V-ATPases function as proton pumps in acidic organelles and plasma membranes of eukaryotic cells. Furthermore, E. hirae V-ATPase physiologically functions as an ion pump, similar to eukaryotic V-ATPases34353637, and is composed of nine subunits with amino acid sequences that are homologous to those of the corresponding subunits of eukaryotic V-ATPases638. Thus, the V1 motor achieves its rotational dynamics via several conformational changes that are generated by the binding of ATP, release of Pi and ADP, and cooperative coupling among these conformational changes.

Next, we soaked the eV1 crystals in a high concentration (2 mM) of ADP to verify nucleotide binding to the third ‘bindable-like' form of 2ADPV1, and obtained the crystal structure (denoted 3ADPV1) at a resolution of 3.0 Å. Three ADP:Mg2+ molecules were bound at all three nucleotide-binding sites and induced conformational changes with the crystal packing rearrangements. We thus designated the unique half-closed AHCBO'' pair of 3ADPV1 as the ‘half-closed' form. A strong electron density peak for Pi or SO42− (a Pi analog) was observed at the nucleotide-binding site with ADP:Mg2+. In contrast, the DF axis and ‘ADP-bound' forms were slightly attracted to the AHC of the ‘half-closed' form. The shifted ‘ADP-bound' form was rather more similar to the observed ‘tight' conformation. We, therefore, designated this shifted ‘ADP-bound' form of 3ADPV1 as the ‘tight-like' form. The distances between the β-phosphate of ADP and the interacting residues in the ‘tight-like' form were slightly longer than those in the ‘ADP-bound' form, suggesting that the binding affinity for ADP of the ‘tight-like' form is lower than that of the ‘ADP-bound' form. Therefore, we inferred that the structure of 3ADPV1 corresponds to the state of waiting for ADP release (that is, ADP-release dwell) in the rotation. The DF axis of 3ADPV1 was slightly bent towards the ‘tight-like' form, but did not induce any rotational changes.

>GSSGSSGMQIGKIIKVSGPLVMAENMSEASIQDMCLVGDLGVIGEIIEMRQDVASIQVYEETSGIGPGEPVRSTGEALSVELGPGIISQMFDGIQRPLDTFMEVTQSNFLGRGVQLPALDHEKQWWFEATIEEGTEVSAGDIIGYVDETKIIQHKIMVPNGIKGTVQKIESGSFTIDDPICVIETEQGLKELTMMQKWPVRRGRPIKQKLNPDVPMITGQRVIDTFFPVTKGGAAAVPGPFGAGKTVVQHQIAKWSDVDLVVYVGCGERGNEMTDVVNEFPELIDPNTGESLMERTVLIANTSNMPVAAREASIYTGITIAEYFRDMGYDVAIMADSTSRWAEALREMSGRLEEMPGDEGYPAYLGSRLAEYYERSGRVIALGSDQREGSITAISAVSPSGGDISEPVTQNTLRVVKVFWGLDSSLAQKRHFPSINWIQSYSLYSTEVGRYMDQILQQDWSDMVTEGMRILQEEEQLNEIVRLVGIDSLSDNDRLTLEVAKSIREDYLQQNAFDDVDTFTSREKQFNMLKVILTFGKEARKALSLGAYFNEIMEGTVAVRERISRSKYIPEEELAKISSINEEIKETIQLIVSEGGMTDD[3x];>GSSGSSGMIKEYRTIKEVVGPLMAVEKVSGVKYEELIEVRMQNGEIRRGQVLEVQEDKAMVQIFEGTSGINLKNSSVRFLGHPLQLGVSEDMIGRVFDGLGRPKDNGPEILPEKYLDINGEVINPIARDYPDEFIQTGISAIDHLNTLVRGQKLPVFSGSGLPHKELAAQIARQATVLDSSDDFAVVFAAIGITFEEAEFFMEDFRQTGAIDRSVMFMNLANDPAIERIATPRMALTAAEYLAYEKGMHVLVIMTDMTNYAEALREISAARREVPGRRGYPGYLYTNLATLFERAGRIRGLKGSVTQIPILTMPEDDKTHPIPDLTGYITEGQIILTRELYKSGIQPPIDVLPSLSRLKDKGTGAGKTREDHAATMNQLFAAYAQGKQAKELAVVLGESALSDIDKIYAKFAERFENEYVNQGFYTNRTITETLDLGWELLAMLPRTELKRIKDDLLDKYLPEGK[3x];> GSSGSSGMRLNVNPTRMELTRLKKQLTTATRGHKLLKDKQDELMRQFILLIRKNNELRQAIEKETQTAMKDFVLAKSTVEEAFIDELLALPAENVSISVVEKNIMSVKVPLMNFQYDETLNETPLEYGYLHSNAELDRSIDGFTQLLPKLLKLAEVEKTCQLMAEEIEKTRRRVNALEYMTIPQLEETIYYIKMKLEENERAEVTRLIKVKNMGTEE;> MTYKIGVVGDKDSVSPFRLFGFDVQHGTTKTEIRKTIDEMAKNEYGVIYITEQCANLVPETIERYKGQLTPAIILIPSHQGTLGIGLEEIQNSVEKAVGQNILSGPSSGENLYFQ>GYQKDIDKVYKEQN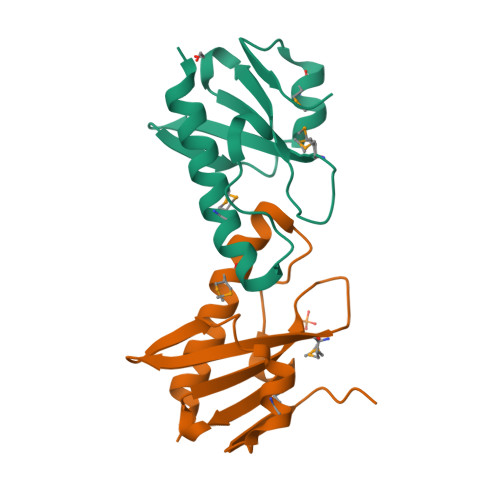QMNKIASKVQNTIKTDIKQEDSNTHVYKDGKVIVIGIQLYKDREKMYYFAYEIKDGKAEINREIDPIKYMKDHKADYEDENVEVEKD[2x]>[2x]THATSTETIHYVNEDG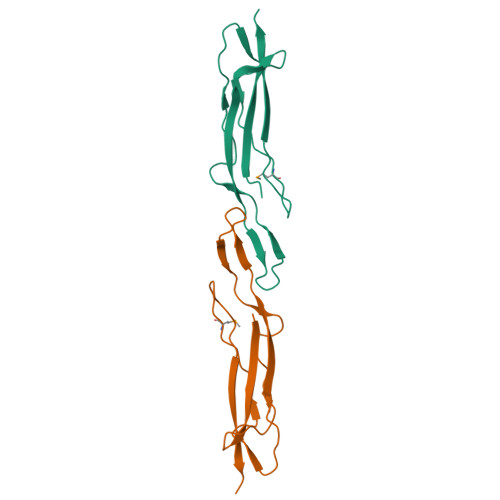DQVFEDGGGKLDFTRTVTIDDVTNEVVEYGEWTPVTDDEFAAVTSPDKDGYTPDTSEVAAQKPDMTDGPDGTVKDVEVTVTYTANPAVATI> MMMKRDYGGVGTIALRASALLKAMSQDIEDQRKEFNQTEYYQTFTRNAVAKLPKLSRRIVDQAIKEMEEDGYQFNKKQVGNVEQYALTIQNVIDIYAHRKIPKYRDIHKSPYVIFVVNLKGGVSKTVSTVTLAHALRVHQDLLRHDLRILVIDLDPQASSTMFLDHTHSIGSILETAAQAMLNNLDAETLRKEVIRPTIVPGVDVIPASIDDGFVASQWRELVEEHLPGQNQYEILRRNIIDRVADDYDFIFIDTGPHLDPFLLNGLAASDLLLTPTPPAQVDFHSTLKYLTRLPEMLEQLEEEGVEPRLSASIGFMSKMTGKRDHETSHSLAREVYASNILDSSLPRLDGFERCGESFDTVISANPQSYPGSAEALKKARTEAERFTKAVFDRIEFV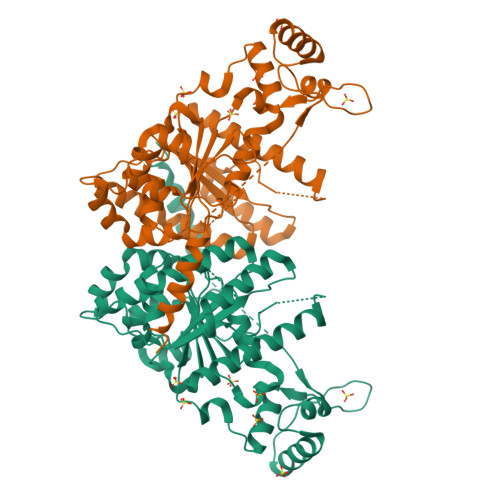RGEAA> GIADGTMLIGDSVALRANTALQTAL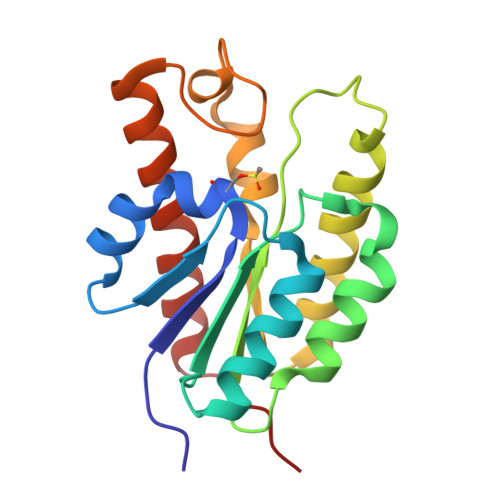PGAQINAQVSVTTKTANEIMLNNSQNKFLPKTVVIATGVNNPENYKDDWDSIVKNLPKGHHMILVTPYEGDKTKETYAIVEKAAAYMRELAEKTPYITIADWNQVAKEHPEIWAGTDQVHFGSESSTIEAGAKLYADTIATALQTAQDKPVKSK>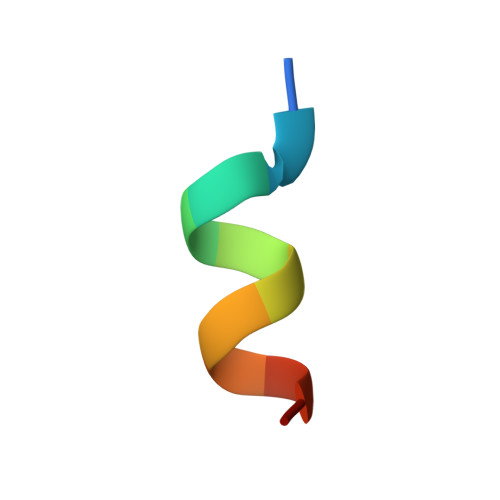 KHKILHRLLQD> GSNRRLQQTQAQVDEVVDIMRVNVDKVLERDQKLSELDDR;> MALSEIETRHSEIIKLENSIRELHDMFMDMAMLVESQGEMIDRIEYNVEHAVDYVERAVSDTKKAVK;> MRNELEEMQRRADQLADESLESTRRMLQLVEESKDAGIRTLVMLDEQGEQLDRVEEGMNHINQDMKEAEKNLKDLGK;> MARENEMDENLEQVSGIIGNLRHMALDMGNEIDTQNRQIDRIMEKADSNKTRIDEANQRATKMLG;> MEFVMKQALGGATKDMGKMLGGDEEKDPDAAKKEEERQEALRQAEEERKAKYAKMEAEREVMRQGIRDKYGIKKKEEREA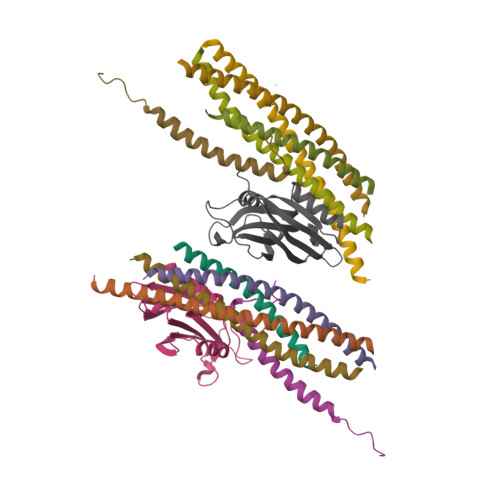EAQ;> QEKLGDICFSLRYVPTAGKLTVVILEAKNLKKMDVGGLSDPYVKIHLMQNGKRLKKKKTTIKKNTLNPYYNESFSFEVPFEQIQKVQVVVTVLDYDKIGKNDAIGKVFVGYNSTGAELRHWSDMLANPRRPIAQWHTLQVEEEVDAMLAVKK> LLDTGEIVPGAFASVKKVGDFPLLPLSLLLSRLKERRQELLRDWQVHAVRQAAVREPLAEATRENDGGAGPRAVEAFAREEERIQRKIKILELLACGGLEENASSQGAIGDAKRIAFLAHADAVNLLLLLAAEAETLARPGEREETEGKEGSSAVGEISKQEERQLWRLKCEGNEEKWNLCISRLKELALDHEDSFLVFYAMCSTNRFDAVLLPALLERLEASFFSSQALSKPLFHPIFEVWDPPCESFAALINVLPLSAKAVVVTADRRSERERRENEGWLAPPEAPPLVLPNWQTMHPVDME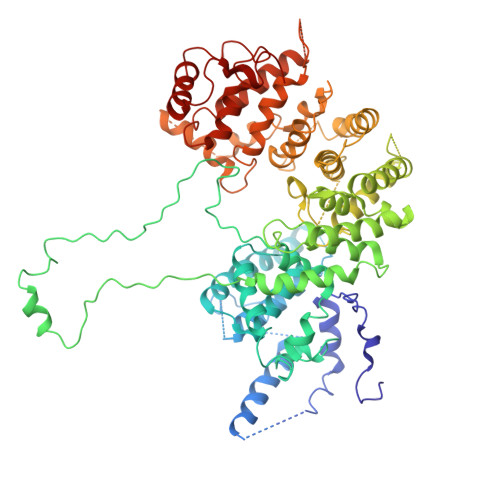AWEKKQRRVVRTRHVKAKIIRQADGRKLAATMALHGRQAIHRDAAVSSLVSVAAMCASNSQRALRGELLPETLNLLAAELLGRSADALSPHLLSLSFLLSQSSVSLTERLFLHLEAVLRGWLEENGFVEKKQTENVDGESKELCTETASEKRRKASEEQLRNLPPGLNVFGLVQSSPSSSDALLASGERSETSKSADTESALWESRVLAALLSSFLRVDDYRPSLDFVLLLSDALRNSLRRTAVLSSASESSAPLAIHEKDVLSLKETGALLSSFATSGYAVPPSLMACLVEHFLYDVDLFLTSSPLSPFASSPSSSSSSAEEAEQLSQSFFCSSRGRATPGDCATLLHSLASPSPLSSERLAAADKAGEQKTANLEKLRFEAMTQAWRLVAPVLHLLQPPCKLLILNSLQTAHAPPDVSSTAFFQRSLETFLRDNPDVDSSLLGSLFGTQGR To our knowledge, the best known system that exemplifies this paradigm is the antibiotic agrocin 84, which penetrates into the cytoplasm of the bacterial pathogen Agrobacterium tumefaciens strain C58 by hijacking the PBP called AccA and its cognate transporter. AccA also plays a key-role in the importation of the characteristic plant tumour-derived compounds such as the opines agrocinopines A and B discovered in 1981 in crown gall tumour tissue. The mature AccA structure is a monomer of 493 residues composed of two lobes, each formed by a central β-sheet flanked by α-helices. We identified the pyranose-2-phosphate-like moiety shared by these two ligands as the key recognition template for AccA.

By the molecular replacement method, we then solved the structure of AccA in complex with agrocin 84 at 2.15 Å resolution. Overall, the ligand bound structures are very similar (average rmsd value of 0.33 Å over 490 Cα atoms) adopting a closed conformation. While Agrocinopine A is fully defined in the electron density maps, the leucine-like moiety of agrocin 84 is mobile. Notably, the electron density maps of agrocin 84 show a D-glucopyranose connected via its C2 carbon to the N6-phosphoramidated TM84 moiety and not a D-glucofuranose connected via a C1-linkage as previously suggested using analytical chemistry approaches that were available at the end of the 1970’s. Our structural work showed that the toxin agrocin 84, composed of a glucose moiety linked at its position 2 to TM84, is recognized through a D-glucopyranose-moiety, whereas only a furanose linked at position 1 form had been previously suggested for the structure of agrocin 84. Moreover, in addition to their pyranose interactions, two of these major residues Asn54 and Ser419 also tightly interact with the phosphate/phosphoramidate groups. In contrast, the sucrose moiety of agrocinopine A and the TM84 part of agrocin 84 make only 3 and 2 polar interactions with AccA, respectively. The sucrose moiety and TM84 occupy a different position in the binding site.

> RRALRLGVNGLPNSLEPVNAISNVGPRIVNQIFDTLIARDFFAKGAPGNAIDLVPALAESWERIDEKSVRFKLRQKVMFHDGVELTADDVAYTFSSERLWGPEAIKKIPLGKSYSLDFDEPVVEDKYTVTLRTKTPSYLIETFVASWMSRIVPKEYYKKLGAVDFGNKPVGTGPYKFVEFVAGDRVVLEANDAYWGPKPTASKITYQIVAEPATRVAGLISGEYDIITTLTPDDIQLINSYPDLETRGTLIENFHMFTFNMNQEVFKDKKLRRALALAVNRPIMVEALWKKQASIPAGFNFPNYGETFDPKRKAMEYNVEEAKRLVKESGYDGTPITYHTMGNYYANAMPALMMMIEMWKQIGVNVVMKTYAPGSFPPDNQTWMRNWSNGQWMTDAYATIVPEFGPNGQVQKRWGWKAPAEFNELCQKVTVLPNGKERFDAYNRMRDIFEEEAPAVILYQPYDVYAARKDVHWKPVSFEMMEFRNNLSFG>[6x]MSLVVFPFKHEHPEVLLHNVRVAAAHPRV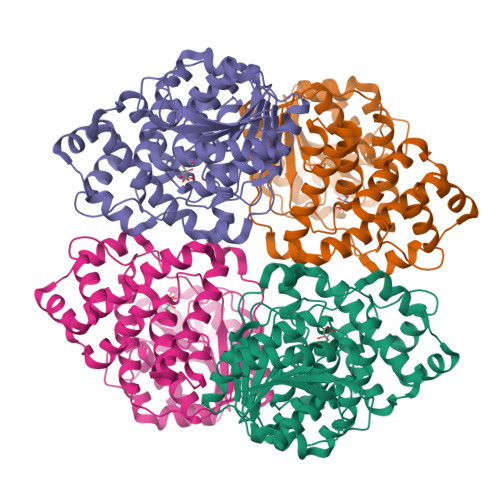HEVLCIGYERDQTYEAVERAAPEISRATGTPVSVRLQERLGTLRPGKGDGMNTALRYFLEETQWERIHFYDADITSFGPDWITKAEEAADFGYGLVRHYFPRASTDAMITWMITRTGFALLWPHTELSWIEQPLGGELLMRREVAAMLYEDERVRRRSDWGIDTLYTFVTVQQGVSIYECYIPEGKAHRLYGGLDDLRTMLVECFAAIQSLQHEVVGQPAIHRQEHPHRVPVHIAERVGYDVEATLHRLMQHWTPRQVELLELFTTPVREGLRTCQRRPAFNFMDEMAWAATYHVLLEHFQPGDPDWEELLFKLWTTRVLNYTMTVALRGYDYAQQYLYRMLGRYRYQAALENGRGHPVPPRAALSTA FLURBIPROFEN METHYL ESTER | C16 H15 F O2 | 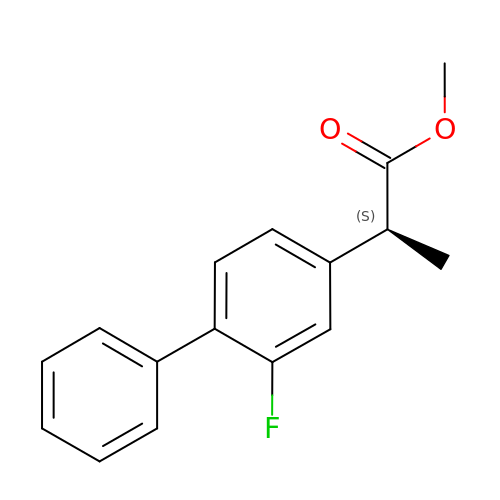CPJBKHZROFMSQM-NSHDSACASA-N>[2x]MGAAILPDLGTEILIPVCAVIGIAFALFQWLLVSKVKLSAVRDASPNAAAKNGYNDYLIEEEEGINDHNVVVKCAEIQNAIS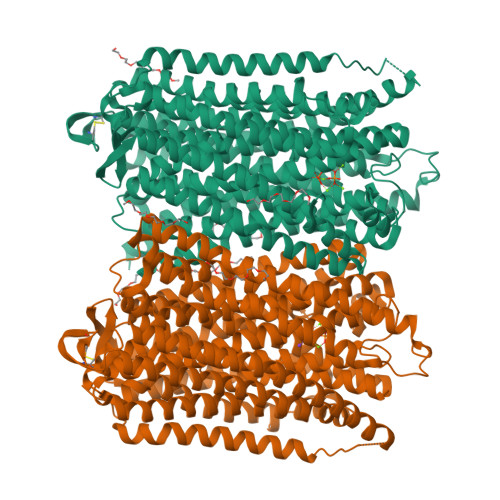EGATSFLFTEYKYVGIFMVAFAILIFLFLGSVEGFSTSPQACSYDKTKTCKPALATAIFSTVSFLLGGVTSLVSGFLGMKIATYANARTTLEARKGVGKAFITAFRSGAVMGFLLAANGLLVLYIAINLFKIYYGDDWGGLFEAITGYGLGGSSMALFGRVGGGIYTKAADVGADLVGKVERNIPEDDPRNPAVIADNVGDNVGDIAGMGSDLFGSYAESSCAALVVASISSFGLNHELTAMLYPLIVSSVGILVCLLTTLFATDFFEIKAVKEIEPALKKQLVISTVLMTIGVAVVSFVALPTSFTIFNFGVQKDVKSWQLFLCVAVGLWAGLIIGFVTEYYTSNAYSPVQDVADSCRTGAATNVIFGLALGYKSVIIPIFAIAISIFVSFTFAAMYGIAVAALGMLSTIATGLAIDAYGPISDNAGGIAEMAGMSHRIRERTDALDAAGNTTAAIGKGFAIGSAALVSLALFGAFVSRASITTVDVLTPKVFIGLIVGAMLPYWFSAMTMKSVGSAALKMVEEVRRQFNTIPGLMEGTAKPDYATCVKISTDASIKEMIPPGALVMLTPLVVGILFGVETLSGVLAGSLVSGVQIAISASNTGGAWDNAKKYIEAGASEHARSLGPKGSDCHKAAVIGDTIGDPLKDTSGPSLNILIKLMAVESLVFAPFFATHGGLLFKIF>MDHLPIFCQLRDRDCLIVGGGDVAERKARLLLEAGARLTVNALTFIPQFTVWANEGMLTLVEGPFDETLLDSCWLAIAATDDDTVNQRVSDAAESRRIFCNVVAAPKAASFIMPSIIDRSPLMVAVSAGGTSPVLARLLREKLESLLPQHLGQVARYAGQLRARVKKQFATMGERRRFWEKFFVNDRLAQSLANADEKAVNATTERLFSEPLDHRGEVVLVGAGPGDAGLLTLKGLQQIQQADIVVYDRLVSDDIMNLVRRDADRVFVGKRAGYHCVPQEEINQILLREAQKGKRVVRLKGGDPFIFGRGGEELETLCHAGIPFSVVPGITAASGCSAYSGIPLTHRDY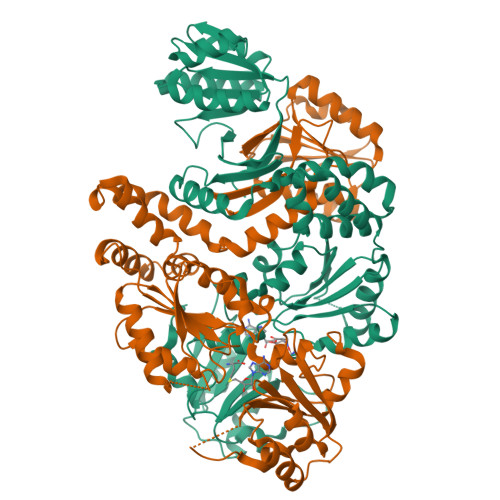AQSVRLVTGHLKTGGELDWENLAAEKQTLVFYMGLNQAATIQEKLIAFGMQADMPVALVENGTSVKQRVVHGVLTQLGELAQQVESPALIIVGRVVALRDKLNWFSNH[2x]> GHMAAAAELSLLEKSLGLSKGNKYSAQGERQIPVLQTNDGPSLMGLTTIAAHLVKQAN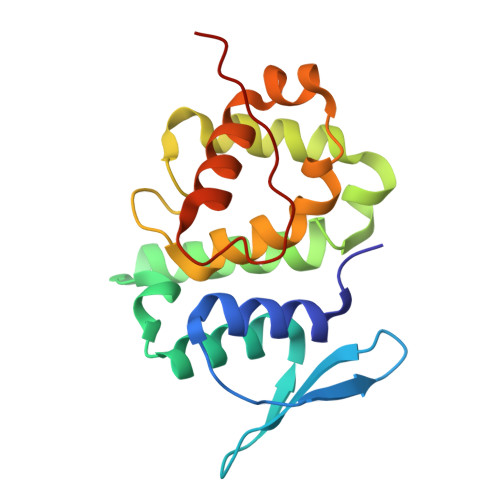KEYLLGSTAEEKAMVQQWLEYRVTQVDGHSSKNDIHTLLMDLNSYLEDKVYLTGYNFTLADILLYYGLHRFIVDLTVQEKEKYLNVSRWFCHIQHYPGIRQHLSSVVFIKNRL> SNAMITKAIYPGTFDPITNGHLDLVT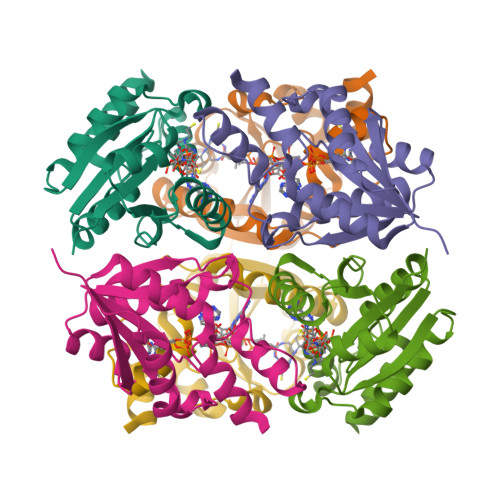RASAMFSHVILAIADSSSKKPMFTLDERVALAKKVTAPLKNVEVLGFSELMAEFAKKHNANILVRGLRSVSDFEYEWQLANMNRHLMPKLESVFLIPSEKWSFISSSLVKEVARHGGDITPFLPKPVTKALLAKLA> MATQHTQYPDARLSSPIVLDQCDLVTRACGLYSSYSLNPQLRNCKLPKHIYRLKYDVTVTKFLSDVPVATLPIDFIVPILLKALSGNGFCPVEPRCQQFLDEIIKYTMQDALFLKYYLKNVGAQEDCVDDHFQEKILSSIQGNEFLHQMFFWYDLAILTRRGRLNRGNSRSTWFVHDDLIDILGYGDYVFWKIPISLLPLNTQGIPHAAMDWYQTSVFKEAVQGHTHIVSVSTADVLIMCKDLITCRFNTTLISKIAEVEDPVCSDYPNFKIVSMLYQSGDYLLSILGSDGYKIIKFLEPLCLAKIQLCSKYTERKGRFLTQMHLAVNHTLEEITEIRALKPSQAHKIREFHRTLIRLEMTPQQLCELFSIQKHWGHPVLHSETAIQKVKKHATVLKALRPIVIFETYCVFKYSIAKHYFDSQGSWYSVTSDRNLTPGLNSYIKRNQFPPLPMIKELLWEFYHLDHPPLFSTKIISDLSIFIKDRATAVERTCWDAVFEPNVLGYNPPHKFSTKRVPEQFLEQENFSIENVLSYAQKLEYLLPQYRNFSFSLKEKELNVGRTFGKLPYPTRNVQTLCEALLADGLAKAFPSNMMVVTEREQKESLLHQASWHHTSDDFGEHATVRGSSFVTDLEKYNLAFRYEFTAPFIEYCNRCYGVKNVFNWMHYTIPQCYMHVSDYYNPPHNLTLENRNNPPEGPSSYRGHMGGIEGLQQKLWTSISCAQISLVEIKTGFKLRSAVMGDNQCITVLSVFPLETDADEQEQSAEDNAARVAASLAKVTSACGIFLKPDETFVHSGFIYFGKKQYLNGVQLPQSLKTATRMAPLSDAIFDDLQGTLASIGTAFERSISETRHIFPCRIT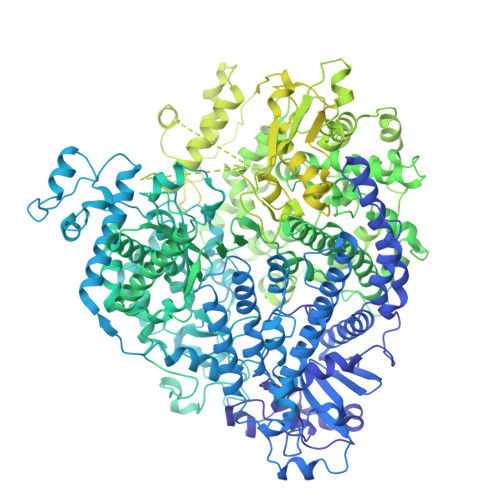AAFHTFFSVRILQYHHLGFNKGFDLGQLTLGKPLDFGTISLALAVPQVLGGLSFLNPEKCFYRNLGDPVTSGLFQLKTYLRMIEMDDLFLPLIAKNPGNCTAIDFVLNPSGLNVPGSQDLTSFLRQIVRRTITLSAKNKLINTLFHASADFEDEMVCKWLLSSTPVMSRFAADIFSRTPSGKRLQILGYLEGTRTLLASKIINNNTETPVLDRLRKITLQRWSLWFSYLDHCDNILAEALTQITCTVDLAQILREYSWAHILEGRPLIGATLPCMIEQFKVVWLKPYEQCPQCSNAKQPGGKPFVSVAVKKHIVSAWPNASRISWTIGDGIPYIGSRTEDKIGQPAIKPKCPSAALREAIELASRLTWVTQGSSNSDLLIKPFLEARVNLSVQEILQMTPSHYSGNIVHRYNDQYSPHSFMANRMSNSATRLIVSTNTLGEFSGGGQSARDSNIIFQNVINYAVALFDIKFRNTEATDIQYNRAHLHLTKCCTREVPAQYLTYTSTLDLDLTRYRENELIYDNNPLKGGLNCNISFDNPFFQGKQLNIIEDDLIRLPHLSGWELAKTIMQSIISDSNNSSTDPISSGETRSFTTHFLTYPKIGLLYSFGAFVSYYLGNTILRTKKLTLDNFLYYLTTQIHNLPHRSLRILKPTFKHASVMSRLMSIDPHFSIYIGGAAGDRGLSDAARLFLRTSISSFLTFVKEWIINRGTIVPLWIVYPLEGQNPTPVNNFLHQIVELLVHDSSRHQAFKTTINDHVHPHDNLVYTCKSTASNFFHASLAYWRSRHRNSNRKDLTRNSSTGSSTNNSDGHIKRSQEQTTRDPHDGTERSLVLQMSHEIKRTTIPQENTHQGPSFQSFLSDSACGTANPKLNFDRSRHNVKSQDHNSASKREGHQIISHRLVLPFFTLSQGTRQLTSSNESQTQDEISKYLRQLRSVIDTTVYCRFTGIVSSMHYKLDEVLWEIENFKSAVTLAEGEGAGALLLIQKYQVKTLFFNTLATESSIESEIVSGMTTPRMLLPVMSKFHNDQIEIILNNSASQITDITNPTWFKDQRARLPRQVEVITMDAETTENINRSKLYEAVHKLILHHVDPSVLKAVVLKVFLSDTEGMLWLNDNLAPFFATGYLIKPITSSARSSEWYLCLTNFLSTTRKMPHQNHLSCKQVILTALQLQIQRSPYWLSHLTQYADCDLHLSYIRLGFPSLEKVLYHRYNLVDSKRGPLVSVTQHLAHLRAEIRELTNDYNQQRQSRTQTYHFIRTAKGRITKLVNDYLKFFLIVQALKHNGTWQAEFKKLPELISVCNRFYHIRDCNCEERFLVQTLYLHRMQDSEVKLIERLTGLLSLFPDGLYRFD>MHHHHHHHDGTENPIHDRTSDYHKYLKVKQGDSDLFKLTVSDKRYIWYNPDPKERDSYECGEIVSETSDSFTFKTVDGQDRQVKKDDANQRNPIKFDGVEDMSELSYLNEPAVFHNLRVRYNQDLIYTYSGLFLVAVNPFKRIPIYTQEMVDIFKGRRRNEVAPHIFAISDVAYRSMLDDRQNQSLLITGESGAGKTENTKKVIQYLASVAGRNQANGSGVLEQQILQANPILEAFGNAKTTRNNNSSRFGKFIEIQFNSAGFISGASIQSYLLEKSRVVFQSETERNYHIFYQLLAGATAEEKKALHLAGPESFNYLNQSGCVDIKGVSDSEEFKITRQAMDIVGFSQEEQMSIFKIIAGILHLGNIKFEKGAGEGAVLKDKTALNAASTVFGVNPSVLEKALMEPRILAGRDLVAQHLNVEKSSSSRDALVKALYGRLFLWLVKKINNVLCQERKAYFIGVLDISGFEIFKVNSFEQLCINYTNEKLQQFFNHHMFKLEQEEYLKEKINWTFIDFGLDSQATIDLIDGRQPPGILALLDEQSVFPNATDNTLITKLHSHFSKKNAKYEEPRFSKTEFGVTHYAGQVMYEIQDWLEKNKDPLQQDLELCFKDSSDNVVTKLFNDPNIASRAKKGANFITVAAQYKEQLASLMATLETTNPHFVRCIIPNNKQLPAKLEDKVVLDQLRCNGVLEGIRITRKGFPNRIIYADFVKRYYLLAPNVPRD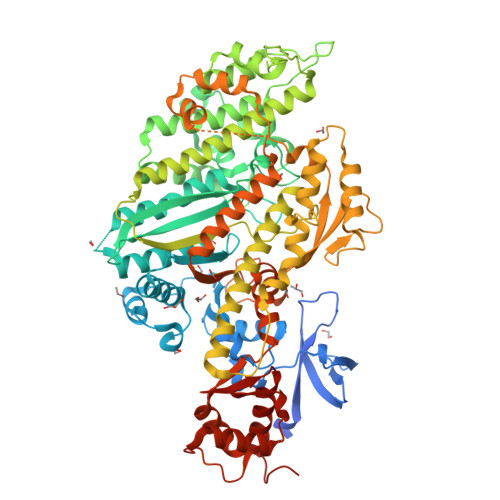AEDSQKATDAVLKHLNIDPEQYRFGITKIFFRAGQLARIEEAREQRLESNEPPMDFDDDIPF[2x]3-[2-[(Z)-[3-(2-carboxyethyl)-5-[(Z)-(3-ethenyl-4-methyl-5-oxo-pyrrol-2-ylidene)methyl]-4-methyl-pyrrol-2-ylidene]methyl]-5-[(Z)-(3-ethenyl-4-methyl-5-oxo-pyrrol-2-ylidene)methyl]-4-methyl-1H-pyrrol-3-yl]propanoic 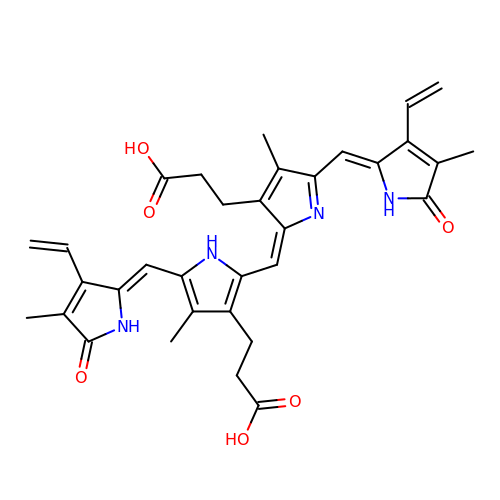acid | C33 H34 N4 O6 | JXYQCWFZZAWTEC-SRVCBVSDSA-N>MAENDFGIAIIGMAGRFPQADTVQAFWENLLASRECISFYSDEELLAMGISPEFVQHPDYVKAKGEVADIDKFDAAFFGIAPREAELMDPQHRVLLETAWAAFEDAGYVAADYPGDVGIFAGKSMDSYLMLNLMPHFKRVFSSGSLQ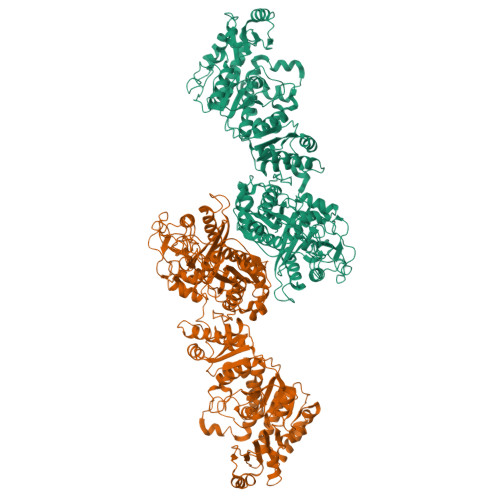AAIGNDKDSITTTIAYHLNLRGPAITVQTSSSTSLVAVCVACQSLLTWQCDMAIAGGVTLGPPAKTGYLSQEGGITAADGHCRAFSDNSSGFVPGTGAGLVVLKRVDEALRDGDNIYAVIKGFAVNNDGSEKISYTAPSVDAQARAIAQAQRLAGLTPQDITYVEAHGTGTRLGDPVEFSALSQAFAGASQKQYCALGSVKTNIGHLDTAAGVAGLIKTALAVQQGIIPATLHFERPNAQIDLTNSPFYINTTCQPWQPESGIRRAGVTSLGMGGTNAHVVLEQAPAVDLQARAPVPAYSILPFSAKTDSALSSGLARFADFLQHESLPDRRDLAWTLSQGRKAFAHRAALVTRDLHAAGTLLQQAATAPFARGVAQTQLGLGLLFSGQGSQYQRMGHQLYQVWPAYADAFDRCATLLEREYQLDIRHELFRAEVSLAQGERLAQTCLTQPLLFSVEYALAQLWLSWGITPTVMIGHSLGEWVAATLAGVFSLEDALRLVARRAELMHQAPSGAMLMVALPEAQIRALITAPLAIAAVNAPDYSVIAGPTSEILAVSQRLTEQNIINKRLHTSHAFHSSMMQDAAQALRQAFENVRLNPPTLTIISTVTGAHVSADTLTTPDYWIEQMLMPVQFSAALQEAQATFDVDFLEIGPGATLTQLTNGHALGDRLAFSSLPAGARSSDEHKHILDTVAALWVRGHNIDLSAFAGEQPRRVSLPTYAFDKIRYWVDSPEEQRSAVTPVADAGSVIPSEPSVRRQPRPAFSVPYAAPESKTQRGLVAICEALLGIDGLGIDDNFFEAGGHSLMLGMLLAQVQERFAVTLSFFDVMEDASVRALAQLVEQEQQDDGGSALAVLVNDMINENSSSVDKLAAALEHHHHHH[2x]> MARSITMQQRIEFGDCDPAGIVWYPNYHRWLDAASRNYFIKCGLPPWRQTVVERGIVGTPIVSCNASFVCTAS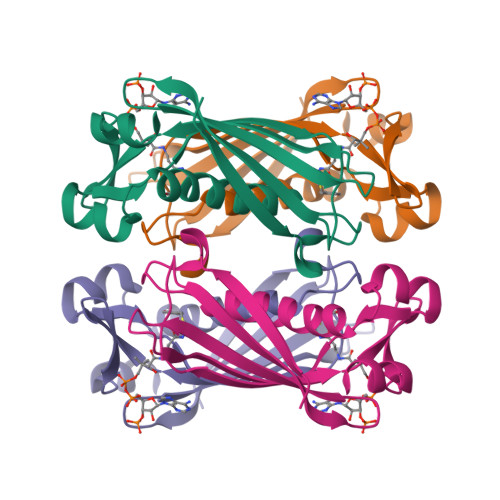YDDVLTIETCIKEWRRKSFVQRHSVSRTTPGGDVQLVMRADEIRVFAMNDGERLRAIEVPADYIELCS N-{[(2R,3R,4R,5R,6S)-3,4,5-trihydroxy-6-methylpiperidin-2-yl]methyl}-1H-indole-2-carboxamide 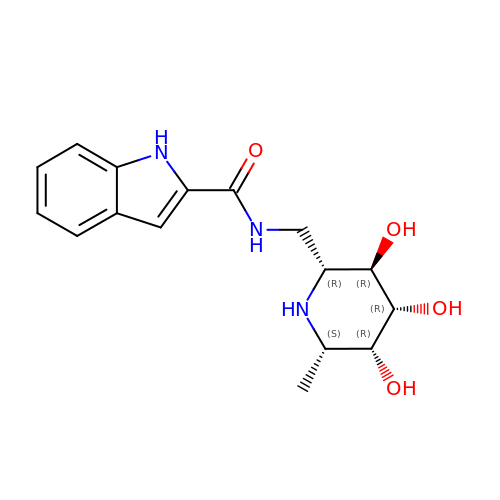| C16 H21 N3 O4 | VHAWVXPAMQXIGT-LMYWXWJPSA-N Aleutian mink disease virus (AMDV), a pathogen in minks, and human parvovirus 4 (PARV4), infecting humans, are parvoviruses belonging to the genera Amdoparvovirus and Tetraparvovirus, respectively. Despite low amino acid sequence identities (10–30%) both viruses share the icosahedral nature of parvovirus capsids, with 60 viral proteins (VPs) assembling the capsid via two-, three-, and five-fold symmetry VP-related interactions, but display major structural variabilities in the surface loops when the capsid structures are superposed onto other parvoviruses. The viral capsids are critical components of the viral infectious life cycle: they protect the viral genome, are the determinants of the tissue type and host that is targeted (tropism), and remain intact while the virus escapes the endo-/lysosomal pathway and trafficks to the nucleus where the genome is released, leading to viral genome replication. The VP monomers of PARV4 and AMDV conserve the β-barrel core motif (βB–βI) with the additional βA strand and the α-helix A (αA) observed in other parvoviruses.

Three-dimensional-image reconstruction of the PARV4 capsids, utilizing a total of 5248 individual particles, resulted in a resolution of 3.12 Å, based on an FSC threshold of 0.143. The reconstructed capsid of PARV4, the first structure of the genus Tetraparvovirus, displayed familiar surface features, similar to those observed in the capsids of other genera in the Parvovirinae subfamily, with channels at the icosahedral five-fold axes, protrusions near the three-fold axes, and depressions at the two-fold axes and surrounding the five-fold axes. Overall, the PARV4 capsid has a “flatter” appearance, similar to some densoviruses, since the three-fold protrusions do not project radially outwards and instead are positioned towards the two-fold, three-fold, and five-fold symmetry axes. This results in very small depressions at the two-fold axes and more segmented depressions surrounding the five-fold channel. While most viruses of the Parvovirinae subfamily possess three separated protrusions surrounding the three-fold symmetry axis, in PARV4, density near the three-fold axis fuses the three-fold protrusions in the shape of a concaved triangle. Structural order in the density map of the PARV4 VP started at lysine 15 (VP2 numbering). The amino acids in the VP monomer were generally well-ordered to the C-terminal leucine 552, with the exception of aa 380–401, located near the three-fold symmetry axis, where only diffuse electron density was observed at a sigma (σ) threshold of ~1, preventing reliable placement of the amino acid chain. The PARV4 capsid utilizes VR-II to form the five-fold channel; VR-I, VR-III, and VR-IX for the two-/five-fold wall; and VR-IV, VR-V, and VR-VIII for the three-fold protrusions. The fused three-fold protrusions are caused by VR-VIII with its subloop leading towards the three-fold symmetry axis.

>[60x]MSVEPAGGGGGVKVKAQWIGGTSFSDSVVITSHTRTSMLADRGGYVPVYKQGSHVDSSQPVMGMKTPYSYIDVNALSAHFTPRDFQQLLDEYDEIKPKSLTIAISAIVIKDVATNQTGTTVSDSASGGITVFADDSYDYPYVLGHNQDTLPGHLPGENYVLPQYGYITRGREIDQQNSIVAISDHKTELFFLEHHDAECLGTGDHWSHHYEFPDDLPWRKLSTPNQTLYARHNPIPSSRLAIMTGVDNDGTAIWKRPEGMDVGRLPLNYVPGPALMMPTDTQIRNTTFRDPVAIGNPATSDRYSVAPLVHQPWSVRTEEWLANKTDYAVHNYLGGVAYTRRKHEESYDKHEEDRDGRVTNPSRVVQIDGDLAAPHVGHTFFVPGHTRVTSGGTDTVYSPKLYQEPVFPLFPGAVWNPNPLSYDCQIWTKIPNTECHFFAQYPLLGGWGVLTPPPMIFVKLRSQPGPPSPGAHTVPQSNLNQYAIFHLHYSMQFLVKRRKRSRRHNPEKPAPFPTTDSGRMPFTLANSLKDPNTPVYEVPSDQWIARNYSHLL>[6x]MKMVVAVIRPEKLECVKKALEERGFVGMTVT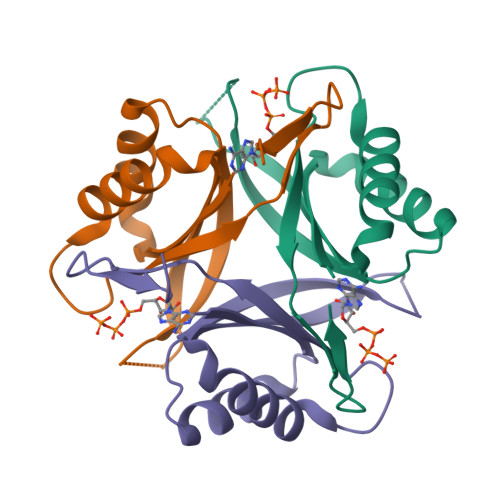EVKGRGEQKGIRLQFRGREVEVDLLQKTKVEVVVSDDAVDEVVEAIVSSARTGKFGDGRIFVIPVEKSVKIRTGDEEVAAAHHHHHH> GSKGDSKETRLTLMEEVLLLGLKDREGYTSFWNDCISSGLRGCMLIELALRGRLQLEACGMRRKSLLTRKVICKSDAPTGDVLLDEALKHVKETQPPETVQNWIELLSGETWNPLKLHYQLRNVRERLAKNLVEKGVLTTEKQNFLLFDMTTHPLTNNNIKQRLIKKVQEAVLDKWVNDPHRMDRRLLALIYLAHASDVLENAFAPLLDEQYDLATKRVRQLLDLDPEVECLKANTNEVLWAVVAA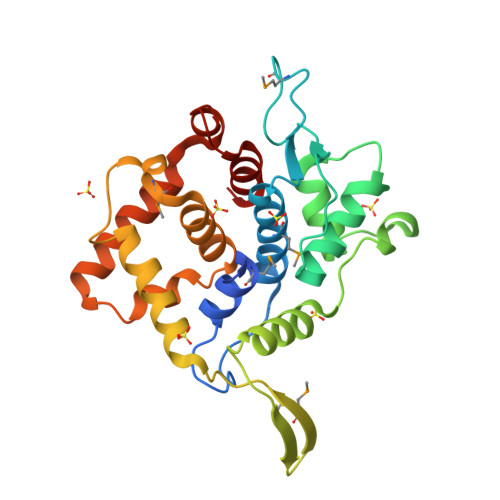FTK>[3x]MGVVREAIAYFAKEAGALSEAELEKVKNGSNEEAIALGEKAVARAKAL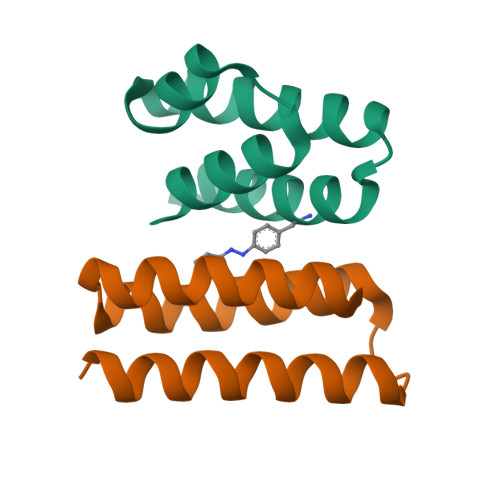GKEKEAKFIKVLVEELKKEGHHHHHH;>MGVEAAKKEIKKLKEEVLKKYKKGEINEEEAIKEFVEKALKLVKAVGDEAVKKFAIEEAKALVEEL[3x]> ADTYAATRYPVILVHGLAGTDKFANVVDYWYGIQSDLQSHGAKVYVANLSGFQSDDGPNGRGEQLLAYVKQVLAATGATKVNLIGHSQGGLTSRYVAAVAPQLVASVTTIGTPHRGSEFADFVQDVLKTDPTGLSSTVIAAFVNVFGTLVSSSHNTDQDALAALRTLTTAQTATYNRNFPSA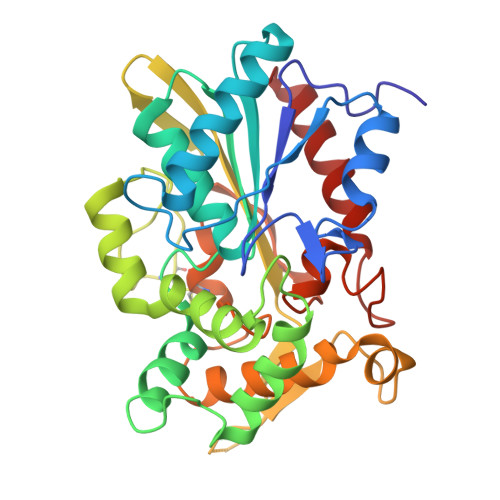GLGAPGSCQTGAATETVGGSQHLLYSWGGTAIQPTSTVLGVTGATDTSTGTLDVANVTDPSTLALLATGAVMINRASGQNDGLVSRCSSLFGQVISTSYHWNHLDEINQLLGVRGANAEDPVAVIRTHVNRLKLQGV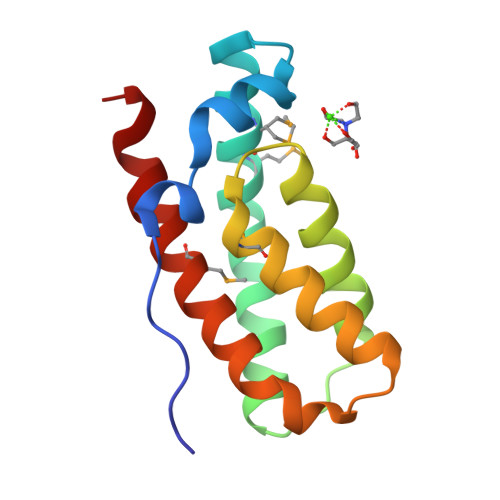> SNAVNEIVVNPNATLDWQLALRQAAGKTDLARDMLQMLLDFLPEVRNKVEEQLVGENPEGLVDLIHKLHGSCGYSGVPRMKNLCQLIEQQLRSGTKEEDLEPELLELLDEMDNVAREASKILG> MAAACAVRGFTTARPMLTPNKVKVPG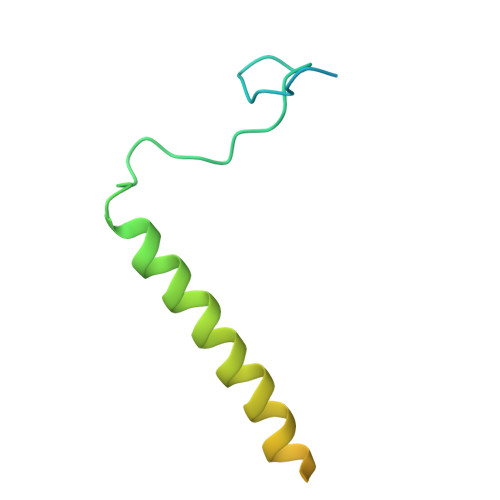RKPQDEEDLTWAEADRKLTPEERYARDKQMALLDKMTSQVEELEKSHTEQKKSNKGVKAQIEAISRQLEALKAQLKE> MAHHHHHHMKLDLKILDARMRDYLPKYATTGSAGLDLRACLDAPVTLKPGDTALVPTGLAIHLADPGYAALILPRSGLGHKHGIVLGNLVGLIDSDYQGELMI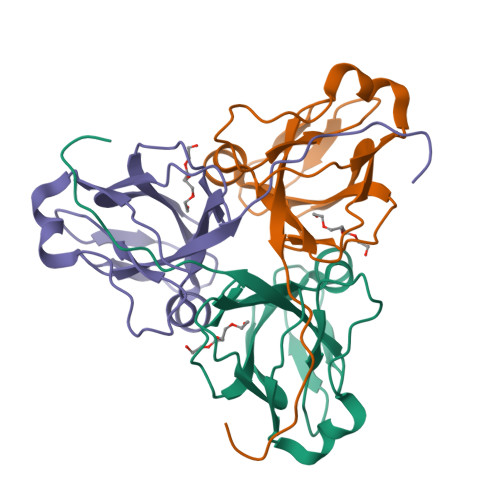STWNRGQTEFVLNPFERLAQLVIVPVVQATFNIVGDFAQSDRGAGGFGSTGRH>[4x]MNHKVHHHHHHIEGRHMEGLLART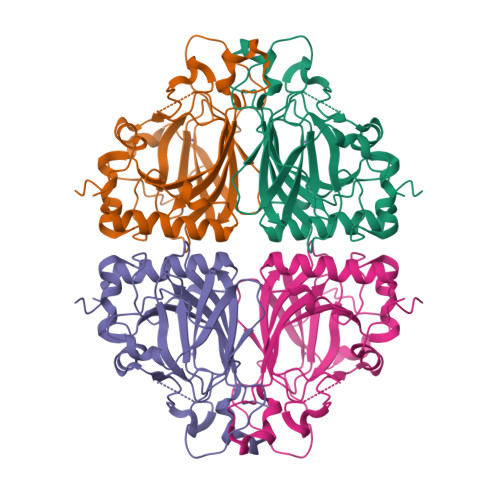SVTRREYDEWLNEAAALGRALRYPVRPEMVNDSAGIVFGEDQYDAFENGLWSREPYEAMVIFESLNEPAVDGLPAAGAPFAEYSGLCDKLMIVHPGKFCPPHYHQRKTESYEVVLGEMELFYSPKPVQVGEEEVLSFTGMHEGSPWPDGVALPIGREESYAALTSYRRLRVGDPKFVMHRKHLHAFRCPADSDVPLVVREVSTYSHEPTEEAADKAAPLPDWAGLHDNSFVAAAANSGRLRTAIQ>[2x]MSPAKEQDRFLPIANVSRIMKRSLPANAKISKEAKETVQECVSEFISFVTGEASDKCQREKRKTINGDDLLWAMTTLGFEAYVGPLKSYLNRYRE;>HM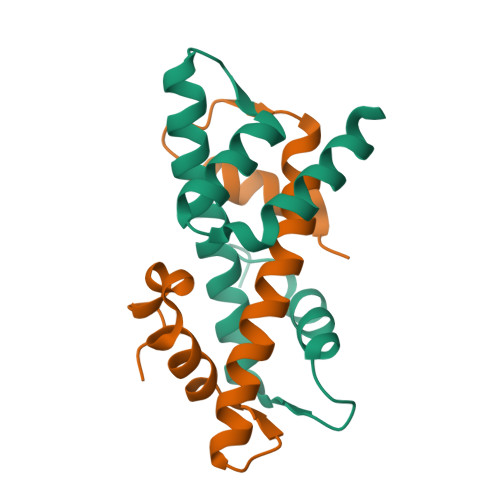QEAERASASDFKNHQLPLARIKKIMKADEDVRMISAEAPVLFAKACELFILELTIRSWLHAEENKRRTLQRNDVAAAIARTDVFDFLVDIVPREEAKEEPGS[2x]Acetylcholine-binding proteins (AChBP) have been described in several gastropods and, more recently, also in an annelid. They are homo-pentamers and water soluble homologues of the extracellular, pentameric ligand-binding domain (LBD) of the membrane-bound nicotinic acetylcholine receptors (nAChR) that belong to the Cys-loop receptor superfamily. In AChBP, the pentameric quaternary structure and the overall subunit features of nAChR-LBD are fully conserved; this also includes the typical pocket-like active site at the five inter-subunit interfaces, with several strictly conserved aromatic residues for ligand binding, and a C-loop for controlled access to the active site. We retrieved full-length sequences of two distinct subunits (termed BgAChBP1 and BgAChBP2), encompassing 205 amino acids plus signal peptide and sharing 52% sequence identity. The resulting cryo-EM structure is a regular pentagonal dodecahedron ∼22 nm in diameter and assembled from twelve ring-like pentamers; each pentamer measures 7–8 nm in height and width and comprises a central channel that is ∼2 nm in diameter.

Recombinant BgAChBP1 formed small particles that we interpreted as pentamers, and much larger particles that are indistinguishable from the native rosette-like protein. We docked twelve copies of the homology-modeled BgAChBP1 pentamer into the 6-Å cryo-EM structure. The correlation coefficient of the fitting was 0.89 as deduced from matching the cryo-EM structure and a density map that was simulated from the molecular model at 6 Å resolution. In addition, BgAChBP1 shows an unprecedented opportunity for a third disulfide bridge, C16↔C64, connecting loops L1 and L3. This bridge is lacking in all other studied members of the Cys-loop receptor superfamily, and it is also absent in BgAChBP2. The potential attachment site in BgAChBP1 for N-linked glycans, N176, is localized next to the C-terminus. The trigonal ring encompasses six different structural elements, each present as three copies: (i) Helix α1 close to the N-terminus of each subunit; (ii) disulfide bridge C16↔C64 that is specific for BgAChBP1 and tethers the C-terminal end of helix α1 to loop L3 of the same subunit; (iii) salt bridge R2↔D26 attaching the N-terminal end of helix α1 to loop L1 of a neighbored subunit from the same pentamer. These specific reinforcements of the N-terminal region of the BgAChBP1 subunit might be required for withstanding the stretching forces inflicted by the other three elements that form the inter-pentamer bridges: (iv) salt bridge D25↔R63 connecting loops L1 and L3 of two subunits from adjacent pentamers; (v) salt bridge R3↔E70 joining the N-terminal end of helix α1 and loop L3 from two subunits of adjacent pentamers; (vi) a central hydrophobic cluster of three F71 residues delivered from three different pentamers. Recombinant BgAChBP1 is able to form a homo-oligomeric dodecahedron, indicating that such a structure also exists within the animal.

>SRRSRSEILQDVLSRCSPLNIPIEDDQPVKVSFEYSLQKIFRADVENDEVDIGLWTTLVWKDRCLNWFNEFTSFKELTVPIAEIWTPDIFIFDSVGAPEIFSDKLARVSQDGTVTYVPQLKVRLSCPLADLKLETGVTCSLKSGSWTHSTQELTLEVNAKVDLGDYASDTRFQLLNATQQVNRKQYPCCPETYEDTTLSFTFRKP[5x]> GMDEKPAITKIISGGQTGADRAALDFAIKHHIPYGGWVPKGRLAEGGRVPETYQLQEMPTSDYSKRTEKNVLDSDGTLIISHGILKGGSALTEFFAEQYKKPCLHIDLDRISIEDAATLINSWTVSHHIQVLNIAG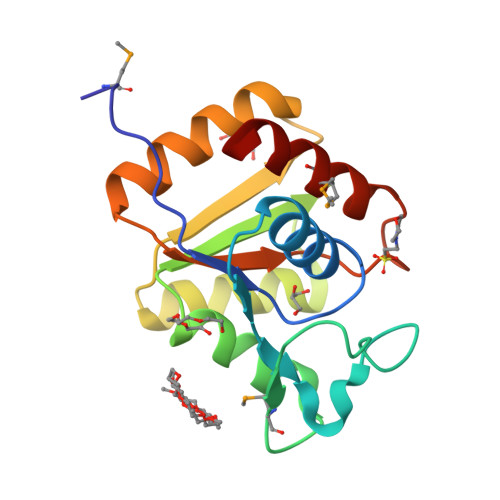PRAGKDPEIYQATMDLLEVFLA>[2x]IREILKMGDE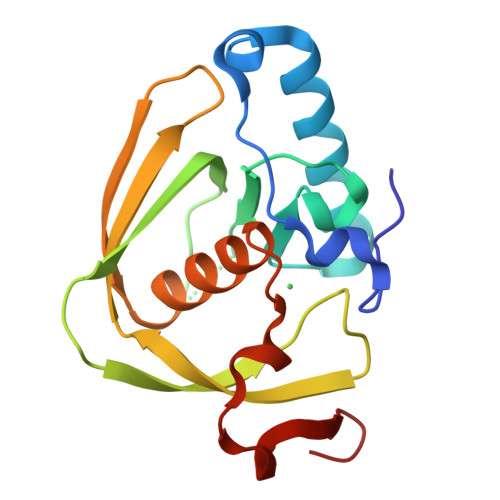RLLRIAQPVPSELLGSEELQRLIDDMFETMHHVGGVGLAAPQIGVDLQLVIFGFERSERYPDAPAVPPTILLNPRITPLDDEMEEGWEGCLSVPGLRGAVSRHRRIRYQGLDPQGQPIDRSVEGFHARVVQHECDHLIGRLYPSRITDFSKFGFTEVLFP>[2x]HHHHHHFNLPPGNYKKPKLLYCSNGGHFLRILPDGTVDGTRDRSDQHIQLQLSAESVGEVYIKSTTGQY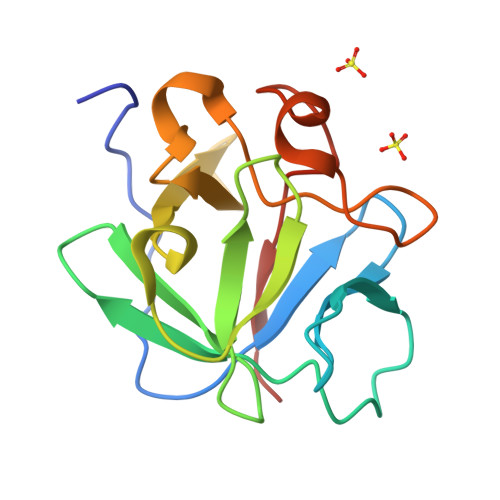LAMDTDGLLYGSQTPNEECLFLERLEENHYNTYISKKHAEKNWFVGLKKNGSCKRGPRTHYGQKAILFLPLPVSSD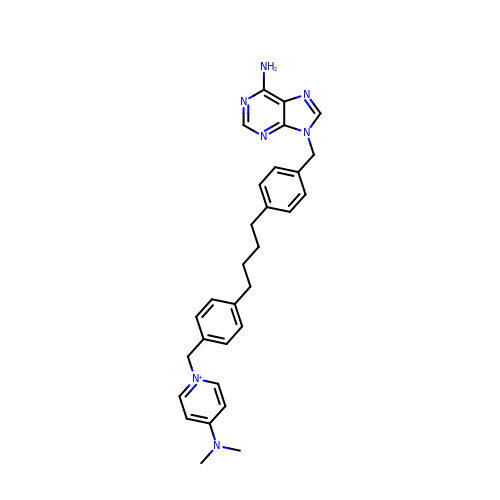1-(4-(4-(4-((6-amino-9H-purin-9-yl)methyl)phenyl)butyl)benzyl)-4- (dimethylamino)pyridinium | C30 H34 N7 | NKYSQEHAAOKBTL-UHFFFAOYSA-N> MSVIQDDYVKQAEQVIRGLPKKNGDFELTTTQLRVLLSLTAQLFDEAQLSSDQNLSPALRDKVQYLRVRFVYQAGREKAVRVFVERAGLLDELAQIGDSRDRL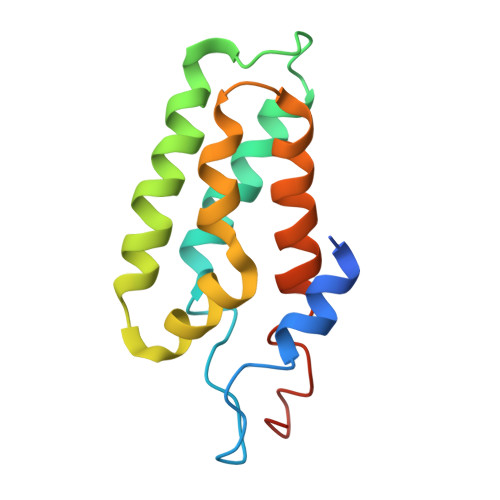LKFCHYMEALVAYKKFLDPKETSKETE> GSVEEKTIKIGFNFEESGSLAAYGTAEQKGAQLAVDEINAAGG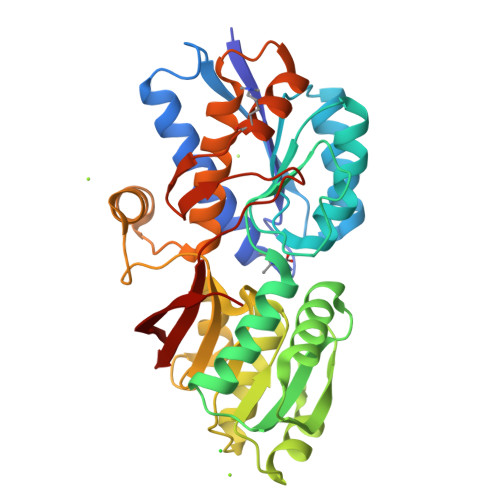IDGKQIEVVDKDNKSETAEAASVTTNLVTQSKVSAVVGPATSGATAAAVANATKAGVPLISPSATQDGLTKGQDYLFIGTFQDSFQGKIISNYVSEKLNAKKVVLYTDNASDYAKGIAKSFRESYKGEIVADETFVAGDTDFQAALTKMKGKDFDAIVVPGYYNEAGKIVNQARGMGIDKPIVGGDGFNGEEFVQQATAEKASNIYFISGFSTTVEVSAKAKAFLDAYRAKYNEEPSTFAALAYDSVHLVANAAKGAKNSGEIKDNLAKTKDFEGVTGQTSFDADHNTVKTAYMMTMNNGKVEAAEVVKP> MENVAEPTVASVSKRIMHNAYYYDKDAKRVGTDSVKRYNSVSVLPNTTTINGKTYYQVVENGKAVDKYINAANIDGTKRTLKHNAYVYASSKKRA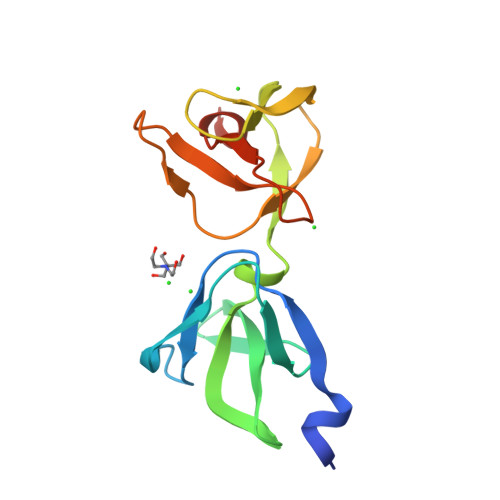NKVVLKKGEVVTTYGASYTFKNGQKYYKIGDNTDKTYVKVANFRLEHHHHH> AGAGAAGGUCUUCUCU

To further understand the structure and properties of the D:U base pair and the D:C mismatch, we designed and synthesized self-complementary RNA sequences that form duplexes with two separated or adjacent D:U or D:C pairs. All four oligonucleotides crystallized within 2–3 days at 20 °C under their optimal crystallization conditions, and we solved their structures by X-ray diffraction at a resolution higher than 1.65 Å. We found that all four structures adopt the same space group (R32). Each unit cell contains only a single RNA strand so that each duplex features two identical D-containing base pairs.

Similarly, the sequence UD-2, 5′-AGA GAA GDU CUU CUC U-3′, can form two adjacent D:U pairs with the underlined nucleobases, while the sequence CD-2, 5′-AGA GAA GDC CUU CUC U-3′, can form two adjacent D:C pairs. Our crystallographic studies show that the D:U base pair has the expected Watson–Crick geometry. Whether separated (UD-1) or adjacent (UD-2) within the RNA duplex, the D:U pairs have identical geometries and exhibit three hydrogen bonds. Relative to a canonical A:U base pair, the third hydrogen bond is between the exocyclic 2-amino group and O2 of U. The H-bond distances between N6–O4, N1–N3, and N2–O2 in both D:U pairs are identical: 2.8, 2.9, and 2.8 Å, respectively. In RNA duplexes, D forms three hydrogen bonds when paired with U, as opposed to two in the A:U pair. This, together with a stronger stacking interaction, results in a D:U base pair being energetically more favorable than an A:U base pair. The larger degree of stabilization is also evidenced by a significant rise in the experimentally determined melting temperature (Tm) of D:U RNA duplexes compared to A:U duplexes. As a result, we observed a 20-fold increase in the binding of the substrate (D*D vs A*A) to a −UU– template.> QVQSVEVMRDSYGVPHVFADSHYGLYYGYGYAVAQDRLFQMDMARRSFVGTTAAVLGPGEQDAYVKYDMQV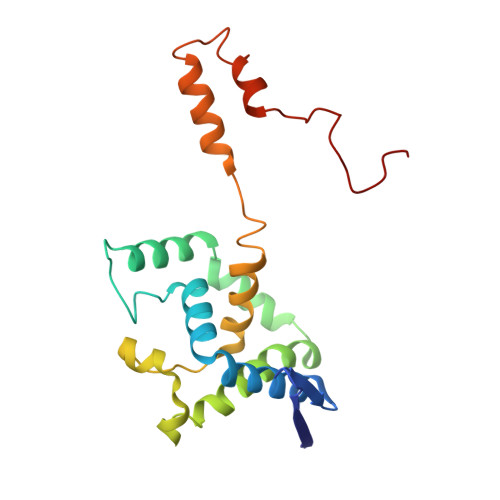RQNFTPASIQRQIAALSKDERDIFRGYADGYNAYLEQVRRRPELLPKEYVDFDFQPEPLTDFDVVMIWVGSMANRFSDTNLEVTALAMRQSLEKQHGPERGRALFDELLWINDTTAPTTVPAPAA> GSGEAEERI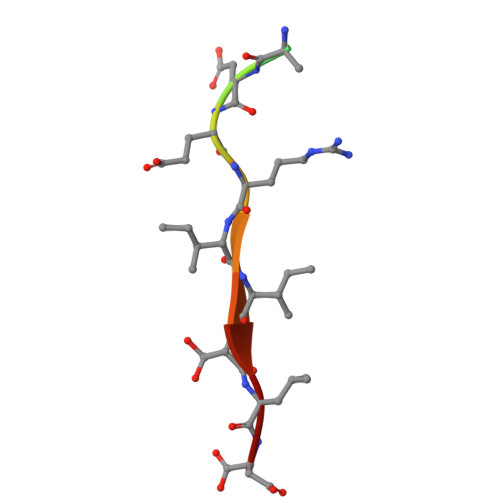ISLD>[2x]SNASSRFSSACIAFIKQWQGLSLEKYRDRQGNWVIGYGHMLTPDE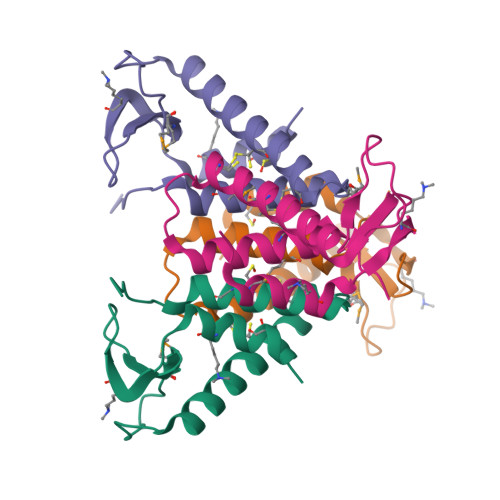TLTFITPDQAEAFLLDDLNSCDILLQNCLPELNDRFQRETLIALMFSIGHQRFLSLINTGD>MIKLYGAPQSRASIIQWYLEELSLPYEFVNVNLKEGEHRQAPYLAINPFGKVPAIADGNFHLWESGAILLYLAEKASTIPADAQARALVNQWILFANSTLANGLFIEAVREKEMPRLLQSLEKILGRSPFILGEKFSVVDVAVGSILAYVPIMLKLNFDDYPAVAAYVQGLVQRPAFQASIGARLEHHHHHH[2x]

Glutathione transferases (GSTs) constitute a widespread superfamily of enzymes notably involved in detoxification processes and/or in specialized metabolism. In the cyanobacterium Synechocsytis sp. PCC 6803, SynGSTC1, a chi-class GST (GSTC), is thought to participate in the detoxification process of methylglyoxal, a toxic by-product of cellular metabolism. GSTCs were shorter of about 30 residues compared to most cytosolic GSTs and had a well-conserved SRAS motif in the active site (10SRAS13 in SynGSTC1). The crystal structure of SynGSTC1 in complex with glutathione adopted the canonical GST fold with a very open active site because the α4 and α5 helices were exceptionally short.

In this study, the crystal structure of the glutathione transferase chi1 from Synechocystis sp. PCC 6803 (SynGSTC1) in complex with GSH is presented. SynGSTC1 crystallized in space group P43212 with two polypeptide chains in the asymmetric unit. They formed a two-fold dimer that had a globular shape with molecular dimensions of approximately 55 Å× 55 Å × 45 Å. The SynGSTC1 protomer adopted the conserved GST fold that was subdivided into two domains for clarity (N-terminal domain β1α1β2α2β3β4α3 and C-terminal domain α4α5α6α7α8). The α4–α5 hairpin pattern was significantly shortened (roughly 10 residues) and the angle between these two helices (~42°) was twice that usually observed. This “missing” region made the active site of SynGSTC1 very open, with no clear pocket for the hydrophobic substrate (H-site). The active site contained GSH tightly bound to the G-site by numerous polar interactions (respectively, six, two and three for the γ-Glu, Cys and Gly moieties). The GSH Cys moiety adopted two rotamers (m, χ1 = −52° and t, χ1 = 172°) exposing the GSH thiol group towards the solvent. The crystal structure did not reveal a strong polar interaction between the sulfur atom of GSH and the enzyme. The Y5 residue, recently proposed as a catalytic residue, was far too distant to stabilize the GSH-thiolate group during catalysis as the Y5 hydroxyl group was 17 Å away from the GSH sulfur-atom.> MASLNTPAPLPTSCNPSDMSHGYVTVKPRVRLHFVELGSGPAVCLCHGFPESWYSWRYQIPALAQAGYRVLAMDMKGYGESSAPPEIEEYCMEVLCKEMVTFLDKLGLSQAVFIGHDWGGMLVWYMALFYPERVRAVASLNTPFIPANPNMSPLESIKANPVFDYQLYFQEPGVAEAELEQNLSRTFKSLFRASDESVLSMHKVCEAGGLFVNSPEEPSLSRMVTEEEIQFYVQQFKKSGFRGPLNWYRNMERNWKWACKSLGRKILIPALMVTAEKDFVLVPQMSQHME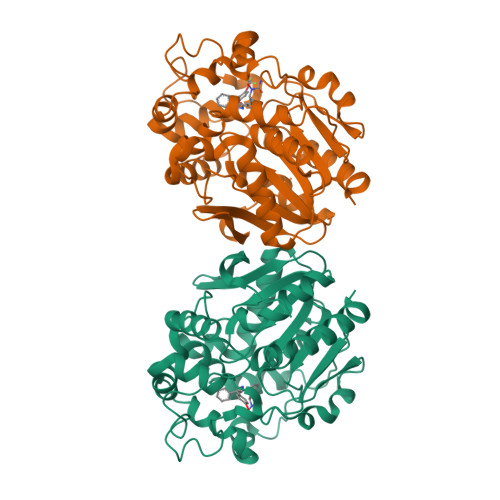DWIPHLKRGHIEDCGHWTQMDKPTEVNQILIKWLDSDARNPPVVSKMLLEHHHHHH TfR1 is a highly recycling receptor expressed on the surface of various cell types, including myofibers and cardiomyocytes, as well as endothelial cells, where it undergoes constitutive endocytosis to transport transferrin-bound ferric ions into the cell. The biological properties of the transferrin receptor make it an ideal candidate for LICA strategies, where conjugation of ASOs and siRNAs to ligands that bind TfR1 promotes their delivery to skeletal and cardiac muscle cells. Bicycle molecules are ∼2-kDa bicyclic peptides formed through the structural constraint of peptides around a trimeric scaffold via formation of thioether cysteine linkages. Here, through effective combination of phage display and peptide medicinal chemistry, we identified and characterized a bicyclic peptide (Bicycle® molecule BCY17901), with a molecular weight of ∼2 kDa, that binds human TfR1 with high affinity and specificity.

Phage selection screens against human TfR1 identified Bicycle molecules that bound to the cognate receptor with sub-micromolar affinity. Subsequent phage display rounds were used to select Bicycle peptides that do not compete with the natural transferrin ligand. Affinity maturation of the lead Bicycle using natural amino acid substitutions was performed to further increase the potency. From this exercise, two Bicycle molecules sharing a common motif were identified for further exploration, BCY15466 and BCY15468 (top two rows). The crystal structure of human His6-TfR1 (called hereafter human TfR1) in complex with the Bicycle molecule BCY15466 was solved at 2.3 Å resolution and used to optimize the binding of the Bicycle lead to TfR1 (see Supplementary Results). An alanine scan was further performed to determine core residues involved in the interaction with the human TfR1 protein and solvent-facing residues that can be used to fine-tune the Bicycle molecular properties such as stability and solubility. Substitution of Ser1, Pro2, and His5 had minimal effect on binding, and the crystal structure showed them to be mostly solvent exposed. Alanine substitution of Leu6 resulted in a small negative effect on binding of ∼5-fold, as measured by fluorescence polarization (FP), which can be explained by the loss of a set of weak intramolecular interactions with the backbone carbonyl of Asp3. Substituting alanine on any of the remaining positions resulted in significant loss of binding, especially Gly3 substitution was highly detrimental to binding because the presence of a glycine in this position permits the turn of loop 1 and is the only compatible residue, since the substitution to Ala or a different side chain would sterically clash with Ser159 of human TfR1. The crystal structure agreed well with the alanine scan data, and molecular interactions could be interrogated to assist in selecting amino acid substitutions to improve Bicycle properties.

> HHHHHHCKGVEPKTECERLAGTESPVREEPGEDFPAARRLYWDDLKRKLSEKLDSTDFTGTIKLLNENSYVPREAGSQKDENLALYVENQFREFKLSKVWRDQHFVKIQVKDSAQNSVIIVDKNGRLVYLVENPGGYVAYSKAATVTGKLVHANFGTKKDFEDLYTPVNGSIVIVRAGKITFAEKVANAESLNAIGVLIYMDQTKFPIVNAELSFFGHAHLGTGDPYTPGFPSFNHTQFPPSRSSGLPNIPVQTISRAAAEKLFGNMEGDCPSDWKTDSTCRMVTSESKNVKLTVSNVLKEIKILNIFGVIKGFVEPDHYVVVGAQRDAWGPGAAKSGVGTALLLKLAQMFSDMVLKDGFQPSRSIIFASWSAGDFGSVGATEWLEGYLSSLHLKAFTYINLDKAVLGTSNFKVSASPLLYTLIEKTMQNVKHPVTGQFLYQDSNWASKVEKLTLDNAAFPFLAYSGIPAVSFCFCEDTDYPYLGTTMDTYKELIERIPELNKVARAAAEVAGQFVIKLTHDVELNLDYERYNSQLLSFVRDLNQYRADIKEMGLSLQWLYSARGDFFRATSRLTTDFGNAEKTDRFVMKKLNDRVMRVEYHFLSPYVSPKESPFRHVFWGSGSHTLPALLENLKLRKQNNGAFNETLFRNQLALATWTIQGAANALSGDVWDIDNEF;> ACPPDAHLGCISWCA>ETGYENTWNFYYERPCCTGNDQGNNNYGKHGADHVREFNCGKLYYRTFHMNEDRDTLYVGAMDRVFRVNLQNISSSNCNRDVINLEPTRDDVVSCVSKGKSQIFDCKNHVRVIQSMDQGDRLYVCGTNAHNPKDYVIYANLTYLPRSEYVIGVGLGIAKCPYDPLDNSTAIYVENGNPGGLPGLYSGTNAEFTKADTVIFRTDLYNTSAKRLEYKFKRTLKYDSKWLDKPNFVGSFDIGEYVYFFFRETAVEYINCGKAVYSRIARVCKKDVGGKNLLAHNWATYLKARLNCSISGEFPFYFNEIQSVYQLPSDKSRFFATFTTSTNGLIGSAVCSFHINEIQAAFNGKFKEQSSSNSAWLPVLNSRVPEPRPGTCVNDTSNLPDTVLNFIRSHPLMDKAVNHEHNNPVYYKRDLVFTKLVVDKIRIDILNQEYIVYYVGTNLGRIYKIVQYYRNGESLSKLLDIFEVAPNEAIQVMEISQTRKSLYIGTDHRIKQIDLAMCNRRYDNCFRCVRDPYCGWDKEANTCRPYELDLLQDVANETSDICDSSVLKKKIVVTYGQSVHLGCFVKIPEVLKNEQVTWYHHSKDKGRYEIRYSPTKYIETTERGLVVVSVNEADGGRYDCHLGGSLLCSYNITV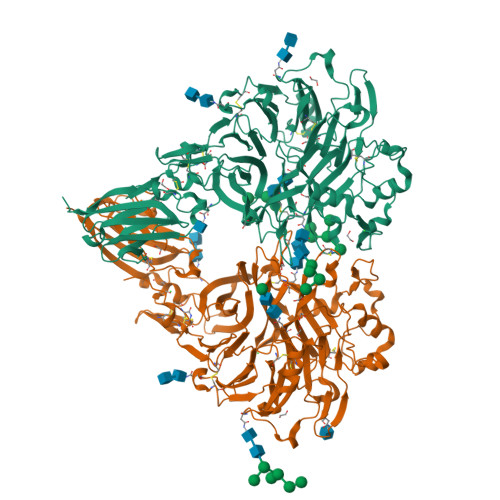DAHRCTPPNKGTKHHHHHH[2x]>MTDTNITTPALTADPEVAAAAAQFLTPVVHKMQALVVNGKQAHWNVRGSNFIAIHELLDSVVAHAQDYADTAAERIVALGLPIDSRVSTMAEKTSTAVPAGFAQWQDEIKAIVSDIDAALVDLQAAIDGLDE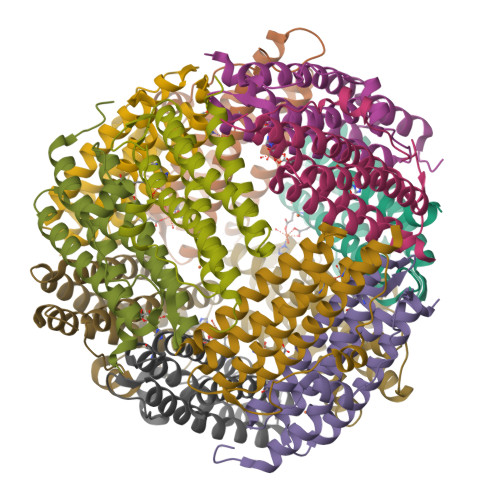VDLTSQDVAIEIKRGVDKDRWFLLAHLAE[12x]> MKKNLLKLTLLLGLAIVLGSCNNEQEKNPQEVNPQTSNDYIIGLIKKCDDCEVSTSKTFFYCGIKAGASYVENDSPYLNDIKESISNGTPIKIYFDENEPERIISVVKISNSEEKNWNLNVKYDETPFKTIEDLNRKVSTQKASSFDFTTTEAVNFFNAMKNKSCAINNQNLCIPFQYANDGCYARAHMMRQ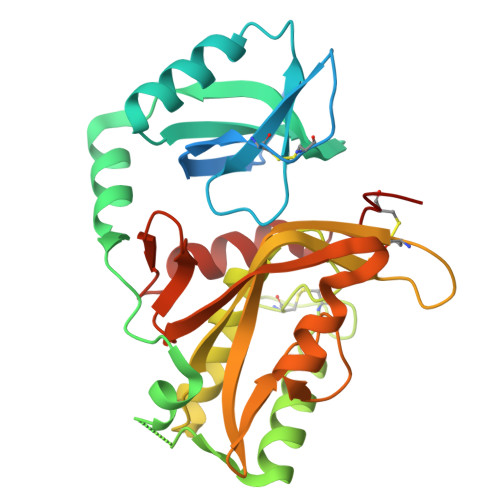HMNYASKDCYKIFAYGNLKVNTSSTGVCGIAWRYHVAPLISVNGVWNVIDPSLFNQPVTITTWLNKMKYNGGTVATTSYQNSSVYYYDYVSNYTQYDNNYTDTYSTLANYRYRQTSCSFL> NEQLAKQKGCMAC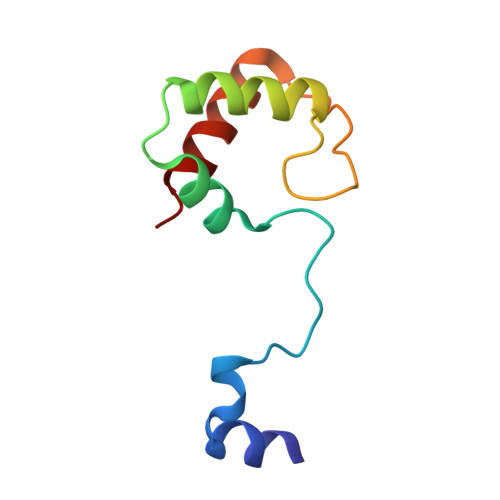HDLKAKMVGPAYKDVAAKFAGQAGAEAELAQRIKNGSQGVWGPIPMPPNAVSDDEAQTLAKWVLSQK>MLRGGVNDCKIKWEFLIGNSIDSSPILAKNGTIYLGSSNKNLYAINTDGSVKWFFKSGEIIECRPSIGKDGTIYFGSDKVYAINPDGTEKWRFDTKKAIVSDFTIFEDILYVTSMDGHLYAINTDGTEKWRFKTKKAIYATPIVSEDGTIYVGS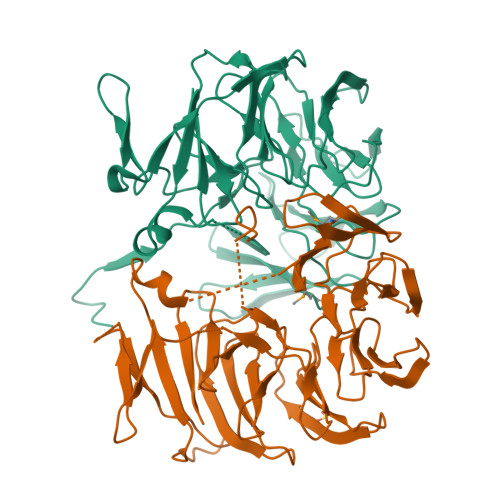NDNYLYAINPDGTEKWRFKTNDAITSAASIGKDGTIYFGSDKVYAINPDGTEKWNFYAGYWTVTRPAISEDGTIYVTSLDGHLYAINPDGTEKWRFKTGKRIESSPVIGNTDTIYFGSYDGHLYAINPDGTEKWNFETGSWIIATPVIDENGTIYFGTRNGKFYALFNLEHHHHHH[4x]> ATAAQAERTLPKKYGGRFTVTLIPGDGVGKEITDSVRTIFEAENIPIDWETINIKQTDHKEGVYEAVESLKRNKIGLKGLWHTPADQTGHGSLNVALRKQLDIYANVALFKSLKGVKTRIPDIDLIVIRENTEGEFSGLEHESVPGVVESLKVMTRPKTERIARFAFDFAKKYNRKSVTAVHKANIMKLGDGLFRNIITEIGQKEYPDIDVSSIIVDNASMQAVAKPHQFDVLVTPSMYGTILGNIGAA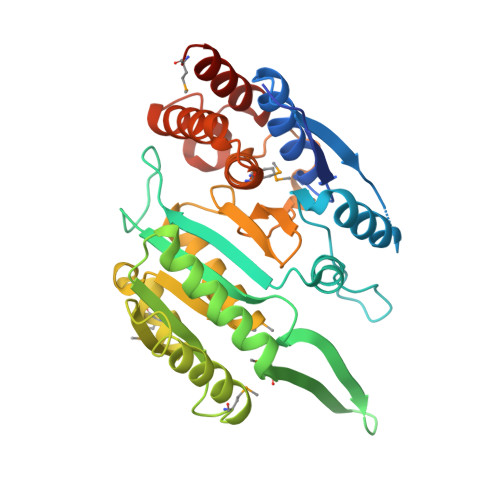LIGGPGLVAGANFGRDYAVFEPGSRHVGLDIKGQNVANPTAMILSSTLMLNHLGLNEYATRISKAVHETIAEGKHTTRDIGGSSSTTDFTNEIINKLSTMHHHHH>MKLIKNGKVLQNGELQQADILIDGKVIKQIAPAIEPSNGVDIIDAKGHFVSPGFVDVHVHLREPGGEYKETIETGTKAAARGGFTTVCPMPNTRPVPDSVEHFEALQKLIDDNAQVRVLPYASITTRQLGKELVDFPALVKEGAFAFTDDGVGVQTASMMYEGMIEAAKVNKAIVAHCEDNSLIYGGAMHEGKRSKELGIPGIPNICESVQIARDVLLAEAAGCHYHVCHVSTKESVRVIRDAKRAGIHVTAEVTPHHLLLTEDDIPGNNAIYKMNPPLRSTEDREALLEGLLDGTIDCIATDHAPHARDEKAQPMEKAPFGIVGSETAFPLLYTHFVKNGDWTLQQLVDYLTIKPCETFNLEYGTLKENGYADLTIIDLDSEQ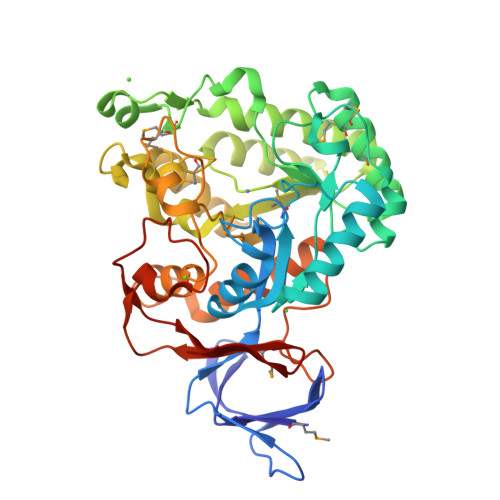EIKGEDFLSKADNTPFIGYKVYGNPILTMVEGEVKFEGDK[2x]>GSAAAQDMVSPPPPIADEPLTVNTGIYLIESYSLDDCAETFKVNAFLSLSWKDRRLAFDPVRSGVRVKTYEPEAIWIPEIRFVNVENARDADVVDISVSPDGTVQYLERFSARVLSPLDFRRYPFDSQTLHIYLIVRSVDTRNIVLAVDLEKVGKNDDVFLTGWDIESFTAVVKPANFALEDRLESKLDYQLRISRQYFSYIPNIILPMLFILFISWTAFWSTSYEANVTLVVSTLIAHIAFNILVETNLPCTPYMTYTGAIIFMIYLFYFVAVIEVTVQHYLKVESQPARA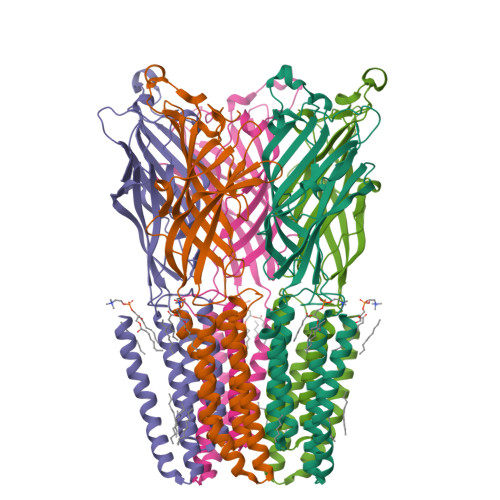ASITRASRIAFPVVFLLANIILAFLFFGF[5x]The fT3SS consists of the transmembrane proteins FlhA, FlhB, FliOPQR, and the soluble ATPase FliI together with its regulators FliJ and FliH (summarized in: Macnab, 2004). FlhB (also: YscU, SpaS, SctU, and Spa40 in the injectisome-related T3SSs; see also: Abrusci et al., 2014) was identified and initially characterized together with FlhA and FlhE in Salmonella enterica. It was shown that FlhB consists of two regions—an N-terminal transmembrane domain (TMD) followed by a cytoplasmic domain (FlhB-C). FlhB-C has the ability for self-cleavage between the asparagine and the proline of the conserved NP(T/E)H motif. Overall, these findings show that FlhB and FliK are important for the switching of the export specificity from rod- and hook-type substrates to filament-type substrates during flagellar morphogenesis.

First, we wished to determine the crystal structure of the cytoplasmic domain of FlhB of the main polar flagellar system [FlhB1 (Sputcn32_2563), henceforth simply FlhB], which localizes at the C-terminus of the protein (SpFlhB-C; amino acid residues: 222–376). The crystal structure of FlhB-C was determined by molecular replacement employing the structure of Salmonella typhimurium FlhB-C as search model, and refined to a resolution of 2.1 Å. All FlhB-C structures share the central domain composed of a four-stranded β-sheet in its center, which is surrounded by four α-helices. Values in parentheses are for highest-resolution shell.As observed for all other FlhB-Cs analyzed so far, autocleavage was also seen in our structure. This autocleavage occurred at the highly conserved 269NPEH272 motif and leads to two tightly associated subdomains FlhB-CN and FlhB-CC (residues 252–269 and 270–376, respectively). However, the structure of SpFlhB-C differs from the other available ones in two main features: First, the N-terminal fraction of helix α1, which connects FlhB-C to its TM domain, appears disordered in our structure. Second, our structure of SpFlhB-C resolves a PRR involving residues 356–376 at the very C-terminus of FlhB-C, which was not observed in previous structures. The PRR follows helix α4 of FlhB-C and appears as a “wave”-shaped linear motif. The PRR interacts with an extended canyon-like surface area formed by helix α4 of FlhB-C. At its C-terminus, the PRR is also in close proximity to helix α3. The interface area between the core domain of FlhB-C and the PRR is 855 Å2 of buried surface area. Our analysis identifies the following hydrogen-bonding pairs between the PRR and helix 4 of the core domain: K360-Y353, G358-Q349, G358-Q352, R359-Q349, R357-Q352, Q368-Q342, and Q368-A339.

>[4x]MGLAQRRMMAEVPNADVIVVNPEHYAVAVKYDVKRSAAPFVIAKGVDDVAFKIREVAREYNIAIVSAPPLARAIYHTTKLDQQIPEGLFTAVAQVLAYVFQLRQYQKGRGRKPIPIPLNQPIPDDLKYHHHHHH>[3x]ENLMQVYQQARLSNPELRKSAADRDAAFEKINEARSPLLPQLGLGADYTYSNGYRDANGINSNATSASLQLTQSIFDMSKWRALTLQEKAAGIQDVTYQTDQQTLILNTATAYFNVLNAIDVLSYTQAQKEAIYRQLDQTTQRFNVGLVAITDVQNARAQYDTVLANELTARNNLDNAVEQLRQITGNYYPELAALNVENFKTDKPQPVNALLK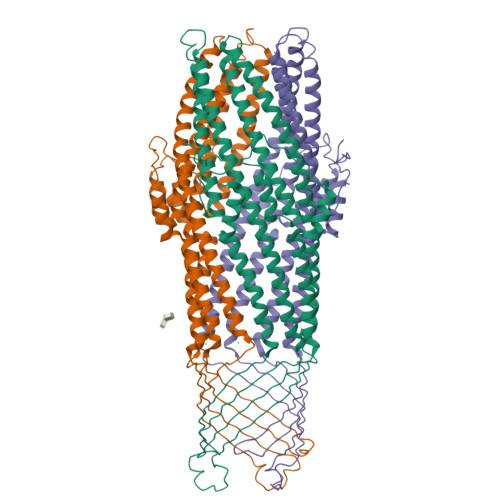EAEKRNLSLLQARLSQDLAREQIRQAQDGHLPTLDLTASTGISDTSYSGSKTRGAAGTQYDDSNMGQNKVGLSFSLPIYQGGMVNSQVKQAQYNFVGASEQLESAHRSVVQTVRSSFNNINASISSINAYKQAVVSAQSSLDAMEAGFSVGTSTIVDVLDATTTLYNAKQELANARYNYLINQLNIKSALGTLNEQDLLALNNALSKPVSTNPE> HHTFEYGDGI;> HHHHHHSSGLVPRGSHMAIYADNSYSIGNTPLVRLKHFGHNGNVVVKIEGRNPSYSVKCRIGANMVWQAEKDGTLTKGKEIVDATS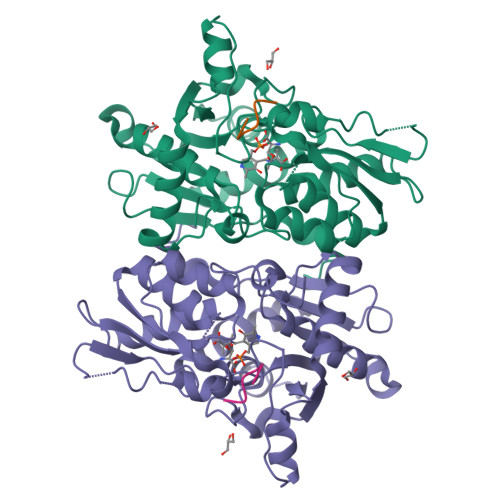GNTGIALAYVAAARGYKITLTMPETMSLERKRLLCGLGVNLVLTEGAKGMKGAIAKAEEIVASDPSRYVMLKQFENPANPQIHRETTGPEIWKDTDGKVDVVVAGVGTGGSITGISRAIKLDFGKQITSVAVEPVESPVISQTLAGEEVKPGPHKIQGIGAGFIPKNLDLSIIDRVETVDSDTALATARRLMAEEGILAGISSGAAVAAADRLAKLPEFADKLIVVILPSASERYLSTALFEGIEG>[2x]MLGAIAYTGNKQSLLPELKSHFPKYNRFVDLFCGGLSVSLNVNGPVLANDIQEPIIEMYKRLINVSWDDVLKVIKQYKLSKTSKEEFLKLREDYNKTRDPLLLYV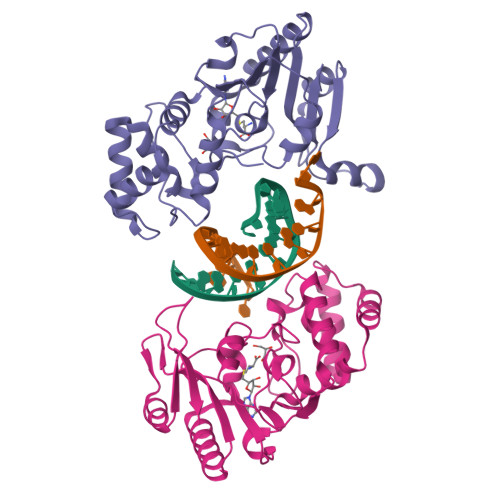LHFHGFSNMIRINYKGNFTTPFGKRTINKNSEKRFNHFKQNCDKIIFSSLHFKDVKILDGDFVYVDPPYLITVADYNKFWSEDEEKDLLNLLDSLNDRGIKFGLSNVLEHHGKENTLLKEWSKKYNVKHLNKKYVFNIYHSKEKNGTDEVYIFN>[2x]MEIEVKFRVNFEDIKRKIEGLGAKFFG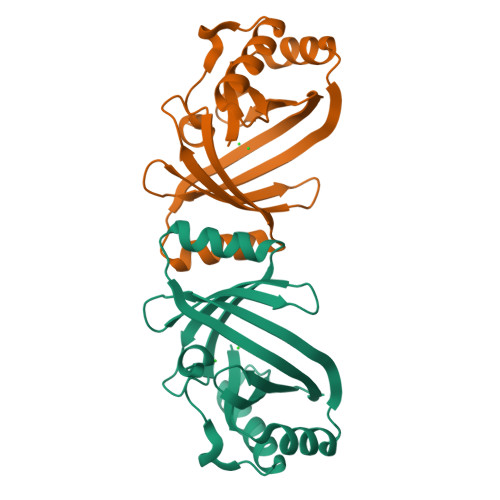IEEQEDVYFELPSPKLLRVRKINNTGKSYITYKEILDKRNEEFYELEFEVQDPEGAIELFKRLGFKVQGVVKKRRWIYKLNNVTFELNRVEKAGDFLDIEVITSNPEEGKKIIWDVARRLGLKEEDVEPKLYIELING> PMF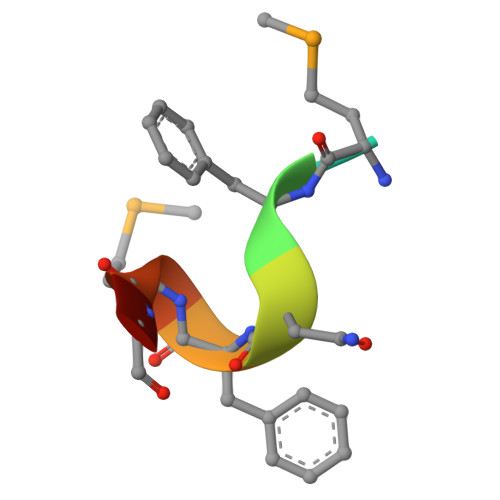NFMGC α-Actinin-2 (ACTN2) is the only muscle isoform of α-actinin expressed in cardiac muscle. All four isoforms of α-actinin consist of an N-terminal actin binding domain (ABD) comprising two calponin homology (CH) domains, connected via a flexible linker, which allows for conformational flexibility in the ABDs, to a rod domain. Thus ACTN2 is important in cross-linking actin and titin filaments in the Z-disc. We have investigated the effects of two mutations identified from HCM patients, A119T and G111V, on the secondary and tertiary structure of a purified actin binding domain (ABD) of ACTN2 by circular dichroism and X-ray crystallography, and show small but distinct changes for both mutations.

G111V was only reported for a 31 year old male, with no family history of HCM. The ABD was in the ‘closed’ conformation in all the structures, as found for other structures of the ABDs for the second striated muscle isoform ACTN3, and the two non-muscle isoforms ACTN1. However, although continuous densities are observed for the loop region at residues 110–120 in both the WT and the A119T mutant structure, this region is disordered for G111V mutant between residues 112 and 117. For both the WT and A119T mutant structure, Val112 is orientated towards the interior of the molecule packing the side chain into a hydrophobic region. For the G111V mutant, the mutant residue Val111 now occupies this same hydrophobic region and thus reorients Val112 and the subsequent residues away from the molecule resulting in a more flexible conformer for this loop region. This larger alteration to the structure for G111V may help to explain the decreased thermal stability for this mutation observed by circular dichroism. The G111V mutation had the greatest effect on stability with its melting temperature (Tm=56.8°C) being 5.5°C lower than that for WT (62.3°C). G111V is just outside of one of these regions, and although this mutation appears to introduce some instability into the subsequent loop containing this binding region, it may not have a large effect on actin binding affinity. The Kd was increased ∼2-fold for the A119T mutant, and ∼1.2-fold for the G111V mutant constructs compared with the WT ABD. After photoactivation of a small region of mEos2-tagged ACTN, we found that the rate of fluorescence decay from the central region of the ‘photoswitched’ area was reduced for both G111V and A119T mutants compared with WT ACTN2, and this change was significant for G111V.

>YMIQEEEWDRDLLLDPAWEKQQRKTFTAWCNSHLRKAGTQIENIEEDFRNGLKLMLLLEVISGERLPKPDRGKMRFHKIANVNKALDYIASKGVKLVSIGTEEIVDGNVKMTLGMIWTIILRFAIQDISVEETSAKEGLLLWCQRKTAPYRNVNIQNFHTSWKDGLGLCALIHRHRPDLIDYSKLNKDDPIGNINLAMEIAEKHLDIPKMLDAEDIVNTPKPDERAIMTYVSCFYHAFAGAEQAETAA[2x]>[2x]MSQTHKHAIPANIADRCLINPEQYETKYKQSINDPDTFWGEQGKILDWITPYQKVKNTSFAPGNVSIKWYEDGTLNLAANCLDRHLQENGDRTAIIWEGDDTSQSKHISYRELHRDVCRFANTLLDLGIKKGDVVAIYMPMVPEAAVAMLACARIGAVHSVIFGGFSPEAVAGCIIDSSSRLVITADEGVRAGRSIPLKKNVDDALKNPNVTSVEHVIVLKRTGSD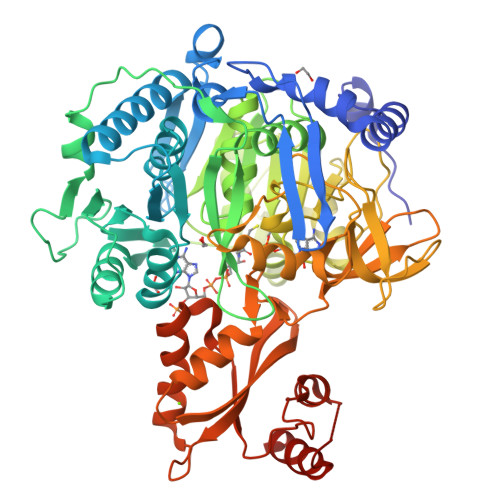IDWQEGRDLWWRDLIEKASPEHQPEAMNAEDPLFILYTSGSTGKPKGVLHTTGGYLVYAATTFKYVFDYHPGDIYWCTADVGWVTGHSYLLYGPLACGATTLMFEGVPNWPTPARMCQVVDKHQVNILYTAPTAIRALMAEGDKAIEGTDRSSLRILGSVGEPINPEAWEWYWKKIGKEKCPVVDTWWQTETGGFMITPLPGAIELKAGSATRPFFGVQPALVDNEGHPQEGATEGNLVITDSWPGQARTLFGDHERFEQTYFSTFKNMYFSGDGARRDEDGYYWITGRVDDVLNVSGHRLGTAEIESALVAHPKIAEAAVVGIPHAIKGQAIYAYVTLNHGEEPSPELYAEVRNWVRKEIGPLATPDVLHWTDSLPKTRSGKIMRRILRKIAAGDTSNLGDTSTLADPGVVEKLLEEKQAIAMPS>[2x]GSPNYDKWEMERTDITMKHKLGGG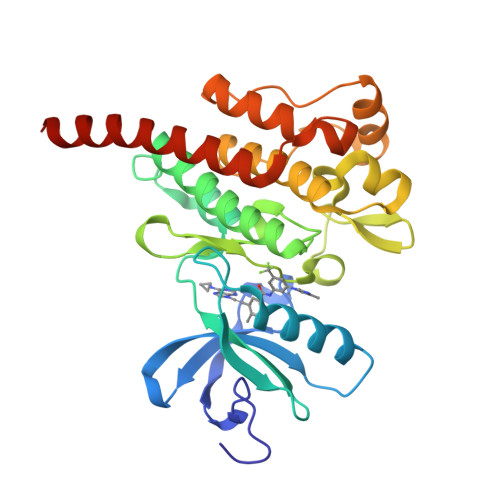QYGEVYEGVWKKYSLTVAVKTLKEDTMEVEEFLKEAAVMKEIKHPNLVQLLGVCTREPPFYIITEFMTYGNLLDYLRECNRQEVSAVVLLYMATQISSAMEYLEKKNFIHRDLAARNCLVGENHLVKVADFGLSRLMTGDTYTAHAGAKFPIKWTAPESLAYNKFSIKSDVWAFGVLLWEIATYGMSPYPGIDLSQVYELLEKDYRMERPEGCPEKVYELMRACWQWNPSDRPSFAEIHQAFETMFQESSISDEVEKELGKRGT> STRRIL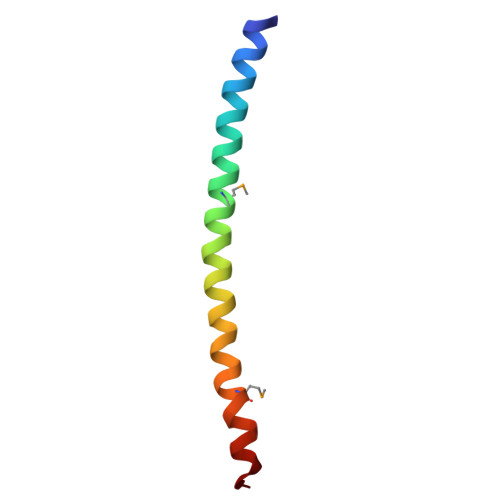GLAIESQDAGIKTITMLDEQKEQLNRIEEGLDQINKDMRETEKTLTEL(2Z)-3-(1H-imidazol-5-yl)-2-iminopropanoic 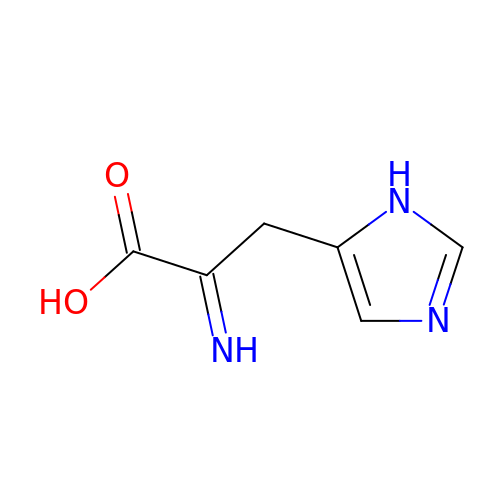acid | C6 H7 N3 O2 | KOGKMQJSUUSGFN-FNORWQNLSA-N> MGSSHHHHHHSSGLVPRGSMSTSWSDRLQNAADMPANMDKHALKKYRREAYHRVFVNRSLAMEKIKCFGFDMDYTLAVYKSPEYESLGFELTVERLVSIGYPQELLSFAYDSTFPTRGLVFDTLYGNLLKVDAYGNLLVCAHGFNFIRGPETREQYPNKFIQRDDTERFYILNTLFNLPETYLLACLVDFFTNCPRYTSCETGFKDGDLFMSYRSMFQDVRDAVDWVHYKGSLKEKTVENLEKYVVKDGKLPLLLSRMKEVGKVFLATNSDYKYTDKIMTYLFDFPHGPKPGSSHRPWQSYFDLILVDARKPLFFGEGTVLRQVDTKTGKLKIGTYTGPLQHGIVYSGGSSDTICDLLGAKGKDILYIGDHIFGDILKSKKRQGWQTFLVIPELAQELHVWTDKSSLFEELQSLDIFLAELYKHLDSSSNERPDISSIQRRIKKVTHDMDMCYGMMGSLFRSGSRQTLFASQVMRYADLYAASFINLLYYPFSYLFRAAHVLMPHESTVEHTHVDINEMESPLATRNRTSVDFKDTDYKRHQLTRSISEIKPPNL

Cytosolic purine 5´-nucleotidase (cN-II; EC 3.1.3.5) dephosphorylates purine nucleotide monophosphates with canonical activity towards inosine monophosphate (IMP). The cN-II protein assembles into functional homotetramers, with each subunit comprising 561 amino acid residues. The cN-II structure possesses the overall fold characteristic of the haloacid dehalogenase superfamily: an α/β Rossmann-like “core domain” and a smaller “cap domain. Whole-exome sequencing studies have recently revealed that somatic missense mutations in the gene encoding cN-II (NT5C2) are associated with relapsed acute lymphoblastic leukemia (ALL).

In this study, we describe the biochemical and structural behavior of the three most common mutants: R367Q, R238W, and L375F. Crystals of all three cN-II mutants belonged to the I222 space group with one molecule per asymmetric unit. Overall, the spatial arrangements of the mutants were almost identical to that of the wild type. The R367Q mutation is located in beta-strand 14 (amino acid residues 367–371) in the proximity of helix A, which is a crucial regulatory segment of cN-II. The replacement of the positively charged arginine residue by a glutamine led to loss of residue 367 hydrogen bonding interactions with both the carbonyl group of S40 and the carboxyl group of D459. Consequently, D459 formed a compensatory polar contact with K361, a residue located in helix A, as illustrated in Fig. 2a. Interestingly, interface A also includes helix A (amino acid residues 355–365), which was well defined in all the mutant crystal structures. Helix A is formed only in the active state of the cN-II enzyme, and the stabilization of this region in the mutants is consistent with their high catalytic potency even in the absence of ATP. In particular, the R367Q variant adopted a fully active conformation that exhibited higher thermostability than the wild-type enzyme.> MEDPDIKRCKLSCVATVDDVIEQVMTYITDPKDRDSASLVCRRWFKIDSETREHVTMALCYTATPDRLSRRFPNLRSLKLKGKPRAAMFNLIPENWGGYVTPWVTEISNNLRQLKSVHFRRMIVSDLDLDRLAKARADDLETLKLDKCSGFTTDGLLSIVTHCRKIKTLLMEESSFSEKDGKWLHELAQHNTSLEVLNFYMTEFAKISPKDLETIARNCRSLVSVKVGDFEILELVGFFKAAANLEEFCGGSLNEDIGMPEKYMNLVFPRKLCRLGLSYMGPNEMPILFPFAAQIRKLDLLYALLETEDHCTLIQKCPNLEVLETRNVIGDRGLEVLAQYCKQLKRLRIERGADEQGMEDEEGLVSQRGLIALAQGCQELEYMAVYVSDITNESLESIGTYLKNLCDFRLVLLDREERITDLPLD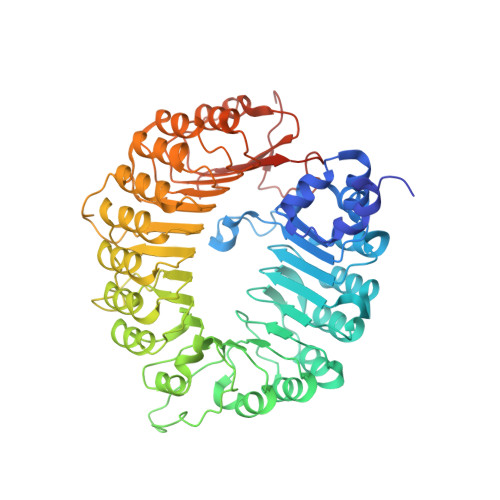NGVRSLLIGCKKLRRFAFYLRQGGLTDLGLSYIGQYSPNVRWMLLGYVGESDEGLMEFSRGCPNLQKLEMRGCCFSERAIAAAVTKLPSLRYLWVQGYRASMTGQDLMQMARPYWNIELIPSRRVPEVNQQGEIREMEHPAHILAYYSLAGQRTDCPTTVRVLKEPI>[4x]ASWSHPQFEKIEGRMQNDILQVVSQGWKYFKGNFYYFSLIPKTWYSAEQFCVSRNSHLTSVTSESEQEF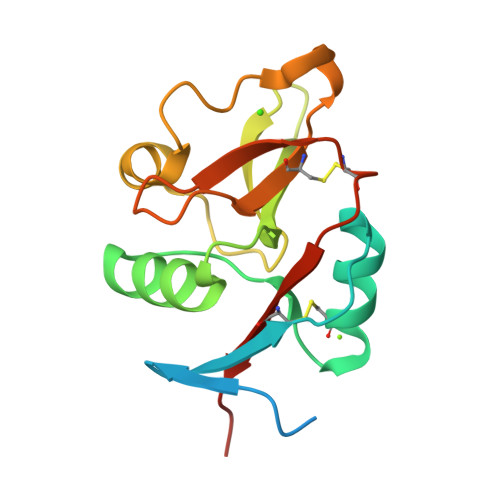LYKTAGGLIYWIGLTKAGMEGDWSWVDDTPFNKVQSARFWIPGEPNNAGNNEHCGNIKAPSLQAWNDAPCDKTFLFICKRPYVPSEP>MSFTPANRAYPYTRLRRNRRDDFSRRLVRENVLTVDDLILPVFVLDGVNQRESIPSMPGVERLSIDQLLIEAEEWVALGIPALALFPVTPVEKKSLDAAEAYNPEGIAQRATRALRERFPELGIITDVALDPFTTHGQDGILDDDGYVLNDVSIDVLVRQALSHAEAGAQVVAPSDMMDGRIGAIREALESAGHTNVRIMAYSAKYASAYYGPFRDAVGSASNLGKGNKATYQMDPANSDEALHEVAADLAEGADMVMVKPGMPYLDIVRRVKDEFRAPT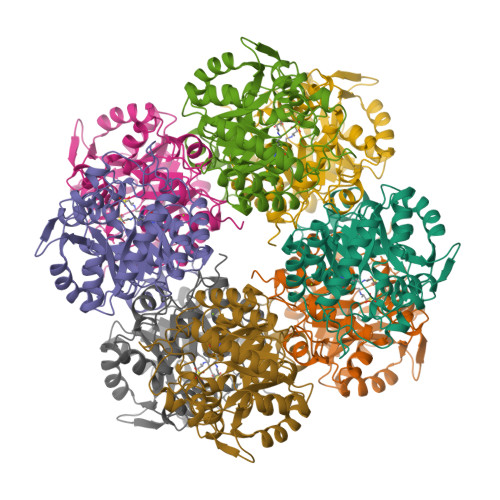FVYQVSGEYAMHMGAIQNGWLAESVILESLTAFKRAGADGILTYFAKQAAEQLRRGR[2x]> SPREQDSESQTLDKVYQMKSKPRGYCLIINNHNFAKAREKVPKLHSI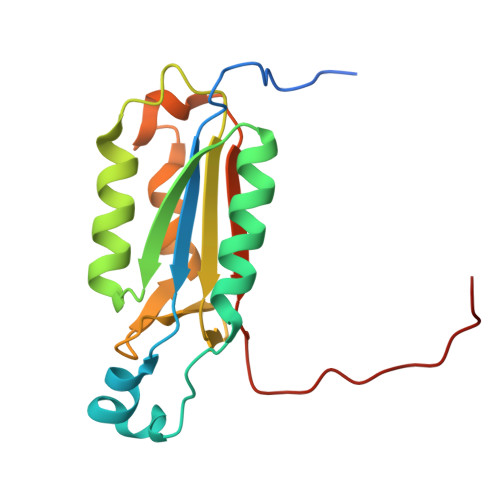RDRNGTHLDAGALTTTFEELHFEIKPHDDCTVEQIYEILKIYQLMDHSNMDCFICCILSHGDKGIIYGTDGQEAPIYELTSQFTGLKCPSLAGKPKVFFIQACQGDNYQKGIPVETD9-{5-O-[(S)-hydroxy{[(R)-hydroxy(phosphonooxy)phosphoryl]oxy}phosphoryl]-beta-D-arabinofuranosyl}-9H-purin-6-amine 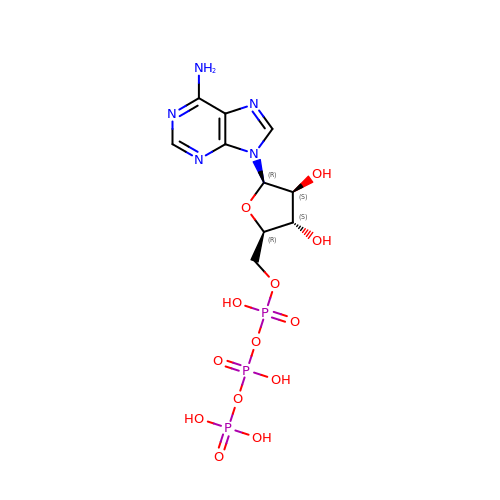| C10 H16 N5 O13 P3 | ZKHQWZAMYRWXGA-UHTZMRCNSA-N2-(CARBAMOYLAMINO)-5-PHENYL-N-[(3S)-PIPERIDIN-3-YL]THIOPHENE-3-CARBOXAMIDE 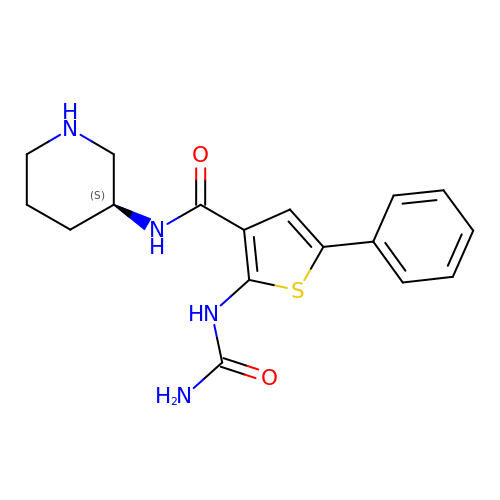| C17 H20 N4 O2 S | UXZRCIBKIDILEF-LBPRGKRZSA-N(2~{S})-4-azanyl-2-[[(2~{S})-4-methyl-2-[[oxidanyl(phenylmethoxycarbonylaminomethyl)phosphoryl]amino]pentanoyl]amino]butanoic 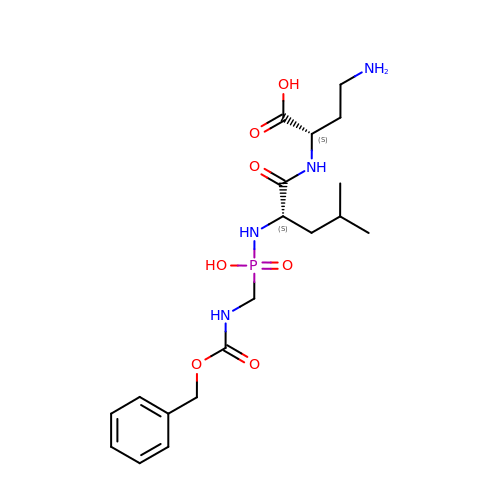acid | C19 H31 N4 O7 P | MUFQKMHBCUDSGW-HOTGVXAUSA-N> MKKCLLFLTTIALILSLSTNAFAKNTSGDLSQKQAL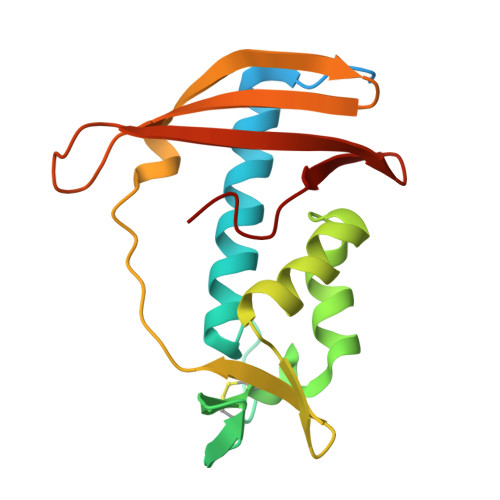QLALSAREHFWNTMSGHNPKVKKAVCPSGTFEYQNLQYVYMCSDLGTKAKAVNYLTPIFTKTAIEKGFKDYHFTVSKGKLAVPIGDGDNLLNWKKSTAKLISKKGSTITYEFTVPTLDGSPSAKRKVTFVKENKKWKVNQFDAVI> GSHMSSLPVPYKLPVSLSTGACVIIKGRPKLSFIN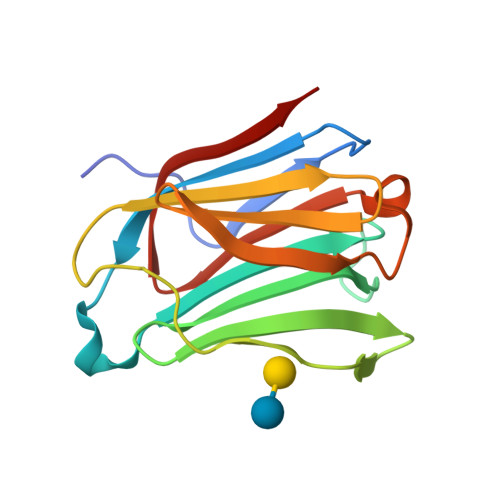DPQLQVDFYTGTDEDSDIAFHFRVHFGHRVVMNSLEFGVWKLEEKIHYVPFEDGEPFELRIYVRHSEYEVKVNGQYIYGFAHRHPPSYVKMIQVWRDVSLTSVCVYN>MKMDKKTIVWFRRDLRIEDNPALAAAAHEGSVFPVFIWCPEEEGQFYPGRASRWWMKQSLAHLSQSLKALGSDLTLIKTHNTISAILDCIRVTGATKVVFNHLYDPVSLVRDHTVKEKLVERGISVQSYNGDLLYEPWEIYCEKGKPFTSFNSYWKKCLDMSIESVMLPPPWRLMPITAAAEAIWACSIEELGLENEAEKPSNALLTRAWSPGWSNADKLLNEFIEKQLIDYAKNSKKVVGNSTSLLSPYLHFGEISVRHVFQCARMKQIIWARDKNSEGEESADLFLRGIGLREYSRYICFNFPFTHEQSLLSHLRFFPWDADVDKFKAWRQGRTGYPLVDAGMRELWATGWMHNRIRVIVSSFAVKFLLLPWKWGMKYFWDTLLDADLECDILGWQYISGSIPDGHELDRLDNPALQGAKYDPEGEYIRQWLPELARLPTEWIHHPWDAPLTVLKASGVELGTNYAKPIVDIDTARELLAKAISRTREAQIMIGA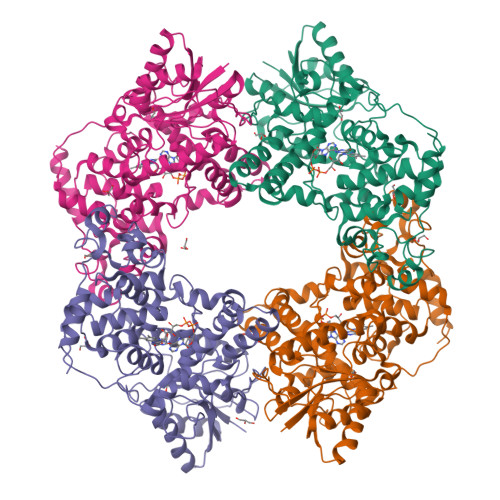A[4x]>[2x]ATCATAWSSSSVYTNGGTVSYNGRNYTAKWWTQNERPGTSDVWADKGACGTGGEGPGGNNGFVVSEAQFNQMFPNRNAFY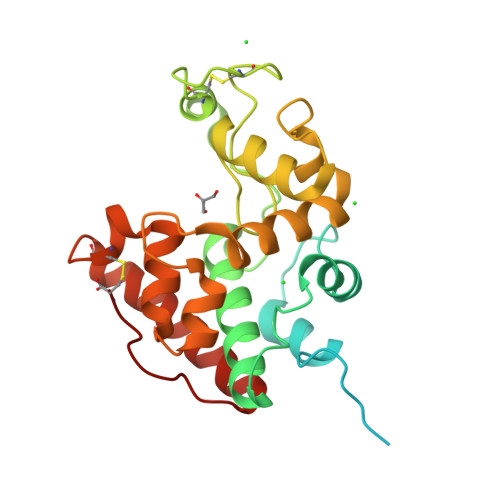TYKGLTDALSAYPAFAKTGSDEVKKREAAAFLANVSHQTGGLFYIKEVNEANYPHYCDTTQSYGCPAGQAAYYGRGPIQLSWNFNYKAAGDALGINLLANPYLVEQDPAVAWKTGLWYWNSQNGPGTMTPHNAIVNNAGFGETIRSINGALECNGGNPAQVQSRINKFTQFTQILGTTTGPNLSC> MVKEDEILPKYWYNIIPDLPKPLPPPRDPQGAYFSRIDLLRSILPKEVL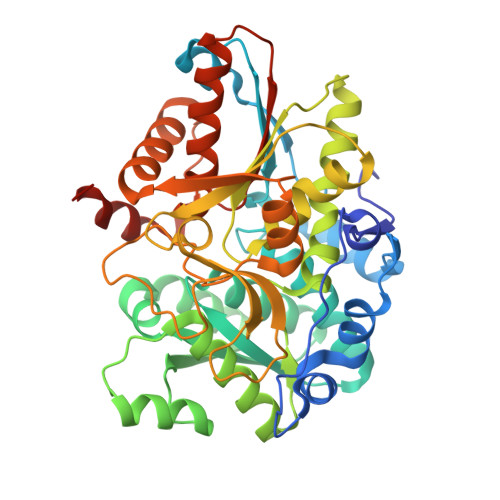RQQFTIERYIKIPEEVRDRYLSIGRPTPLFRAKRLEEYLKTPARIYFKYEGATPTGSHKINTAIPQAYFAKEEGIEHVVTETGAGQWGTAVALAASMYNMKSTIFMVKVSYEQKPMRRSIMQLYGANVYASPTNLTEYGRKILETNPQHPGSLGIAMSEAIEYALKNEFRYLVGSVLDVVLLHQSVIGQETITQLDLLGEDADILIGCVGGGSNFGGFTYPFIGNKKGKRYIAVSSAEIPKFSKGEYKYDFPDSAGLLPLVKMITLGKDYVPPPIYAGGLRYHGVAPTLSLLTKEGIVEWREYNEREIFEAAKIFIENQGIVPAPESAHAIRAVVDEAIEARKNNERKVIVFNLSGHGLLDLSNYESMMKRLNGNG>[8x]MIRIENLSVSYKETLALKDISLVLHGPTITGIIGPNGAGKSTLLKGMLGIIPHQGQAFLDDKEVKKSLHRIAYVEQKINIDYNFPIKVKECVSLGLFPSIPLFRSLKAKHWKKVQEALEIVGLADYAERQISQLSGGQFQRVLIARCLVQEADYILLDEPFAGIDS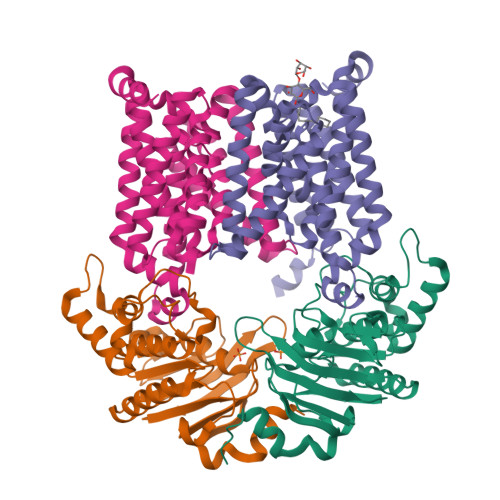VSEEIIMNTLRDLKKAGKTVLIVHHDLSKIPHYFDQVLLVNREVIAFGPTKETFTETNLKEAYGNQLFFNGGDL;>[8x]MIAEFIDGLQKFHFLQNALITAIVVGIVAGAVGCFIILRGMSLMGDAISHAVLPGVALSFILGLDFFIGAIVFGLLAAIIITYIKGNSIIKSDTAIGITSSSFLALGIILIGVAKSSTDLFHILFGNILAVQDTDMFITMGVGAAILLLIWIFFKQLLITSFDELLAKAMGMPVNFYHYLLMVLLTLVSVTAMQSVGTILIVAMLITPAATAYLYANSLKSMIFLSSTFGATASVLGLFIGYSFNVAAGSSIVLTAASFFLISFFIAPKQRYLKLKNKHLLKGSENLYFQ>[2x]MEL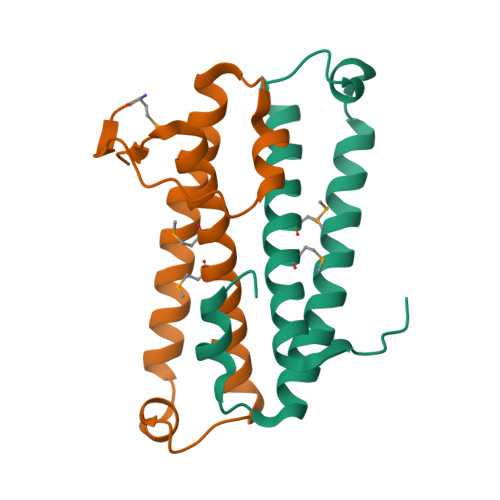EDANVTKKVELRPLIGLTRGLPPTDLETITIDAIRTHRRLVEKADELFQALPETYKTGQACGGPQHIRYIEASIEMHAQMSALNTLYSILGFIPKVVVN> MVSRIICFTLVLVTVVALSYGAAGRESSGGQKWRWGWDPLIRSPVDAEQEVDEQMTNGTKWAVLVAGSKGYGNYRHQADVCHAYQVLKKGGLKDENIVVFMYDDIAKSEMNPRPGIIINSPKGEDVYAGVPKDYTGKNVTVDNLSAVLLGDRSAVKGGSGKVVDSKPEDRIFLFYSNHGGPGVLGMPNEPHLVAKDLVDVLKKKHAMGTYKEMVIYLEACESGSIFEGILPEDLNIYATTASGAQENSYGTYCPGTEPSPPPEYITCLGDLYSVAWMEDSETHNLKKESLEQQFNKVKKRTSNSNTYNTGSHVMEYGSKDIKPEKVYLYLGFDPATVNLPANQIHFDKLDGVNQRDADLIFLWQRYKKSSESTRPEILREITETLTHRGHLDSSIDMIGVLLFGPQNGRSTLHSARAPGLPLVDDWECFKSTARLFEKHCGLLTQYGMKHMRAFANICNSSVEKSKVEEVFIATCGGKNIGPYGTFGAYSV

Asparaginyl endopeptidases (AEPs) are a group of asparagine/aspartic acid (Asx) specific proteases that have been classified as belonging to the C13 family of cysteine proteases based on the presence of a His-Gly-spacer-Ala-Cys motif. First described in plants as vacuolar processing enzymes based on their propensity for processing seed proteins stored in vacuoles, AEPs have since been described in a variety of organisms and shown to be involved in a wide range of processes including, cell death antigen processing and hemoglobin degradation. The recent discovery that evolutionarily distinct plant families have repeatedly recruited AEPs to catalyze the formation of ribosomally synthesized and post-translationally modified peptides (RiPPs), through the macrocyclization of linear precursor sequences, has caught the attention of drug designers keen to overcome the current inefficiencies in native chemical ligation that limit the therapeutic use of cyclic peptides. Herein, we describe the first structure of an active plant AEP; one capable of performing peptide macrocyclization. This AEP, the most abundant AEP of five AEPs in the common sunflower (HaAEP1), displays structural similarity to previously published active AEPs from mammals, with subtle differences at residues involved in substrate recognition.

The crystal structure was solved by molecular replacement yielding a single monomer in the asymmetric unit, and revealed an active monomeric HaAEP1 (residues 58–338 with weak electron density for Asn338) that forms a canonical C13 caspase structure, with a central six-stranded β-sheet region confined by five α-helices. The structure of HaAEP1 lacks the C-terminal cap domain and N-terminal His-Tag, displaying dimensions of approximately 44 Å x 42 Å x 39 Å. The 1.8 Å resolution of our HaAEP1 structure allowed us to observe a succinimide moiety (Snn) below the catalytic His in a location identical to human AEP that was hypothesized to play a role in peptide ligation. We distinguished dual conformations of the catalytic His178 and Cys220 residues which we hypothesize represent conformational changes that occur during catalysis and correspond to substrate free and reaction intermediate states. Close examination of the electron density in the active site of HaAEP1 suggested a small peptide chain is intermittently bound to the intermediate conformation of Cys220. Given AEPs specificity for Asx and the nature of the electron density, we built and refined a tetrahedral complex of a three-residue peptide ligand (AAN) bound to the active site Cys of HaAEP1 with partial occupancy. Residues Ala-Ala were modeled upstream of the P1 Asn due to the weak electron density away from the peptide backbone at these residues.> GTSMETFDPTELPELLKLYYRRLFPYSQYYR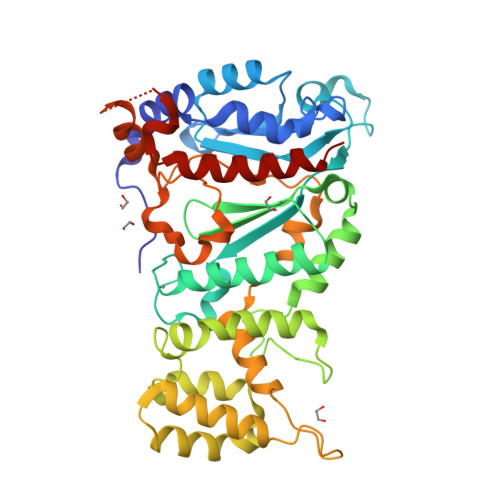WLNYGGVIKNYFQHREFSFTLKDDIYIRYQSFNNQSDLEKEMQKMNPYKIDIGAVYSHRPNQHNTVKLGAFQAQEKELVFDIDMTDYDDVRRCCSSADICPKCWTLMTMAIRIIDRALKEDFGFKHRLWVYSGRRGVHCWVCDESVRKLSSAVRSGIVEYLSLVKGGQDVKKKVHLSEKIHPFIRKSINIIKKYFEEYALVNQDILENKESWDKILALVPETIHDELQQSFQKSHNSLQRWEHLKKVASRYQNNIKNDKYGPWLEWEIMLQYCFPRLDINVSKGINHLLKSPFSVHPKTGRISVPIDLQKVDQFDPFTVPTISFICRELDAISTNEEEKEENEAESDVKHRTRDYKKTSLAPYVKVFEHFLENLDKSRK1-(3,4-dichlorobenzyl)-8-(((1R,4R)-4-hydroxycyclohexyl)amino)-3,7-dimethyl-3,7-dihydro-1H-purine-2,6-dione | C20 H23 Cl2 N5 O3 | 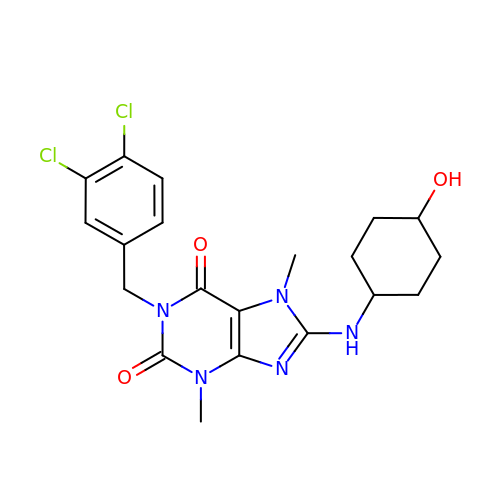AZJJYZNRPSOHRZ-JOCQHMNTSA-N> GVDNAEKGKVSNDDASVDFVAEPVKLPENQTRVAFFYDRAVPIGMLRPGQNMETTFNYQENDYRLNCLLLTPLPSFCPDSSSGPQKTKAPVQWRWVRSGGVNGANFPLMTKQDYAFLCFSPFTFYKCDLEVTVSALGTDTVASVLRWAPTGAPADVTDQLIGYTPSLGETRNPHMWLVGAGNSQVSFVVPYNSPLSVLPAAWFNGWSDFGNTKDFGVAPNADFGRLWIQGNTSASVRIRYKKMKVFCPRPTLFFPWPTPTTTKINADNPVPILELE;> DQNTEEMENLSDRVASDKAGNSATNTQSTVGRLCGYGKSHHGEHPASCADTATDKVLAAERYYTIDLASWTTSQEAFSHIRIPLPHVLAGEDGGVFGATLRRHYLCKTGWRVQVQCNASQFHAGSLLVFMAPEFYTGKGTKTGTMEPSDPFTMDTEWRSPQGAPTGYRYDSRTGFFATNHQNQWQWTVYPHQILNLRTNTTVDLEVPYVNVAPSSSWTQHANWTLVVAVLSPLQYATGSSPDVQITASLQPVNPVFNGLRHETVIAQ;> SPIPVTVREHK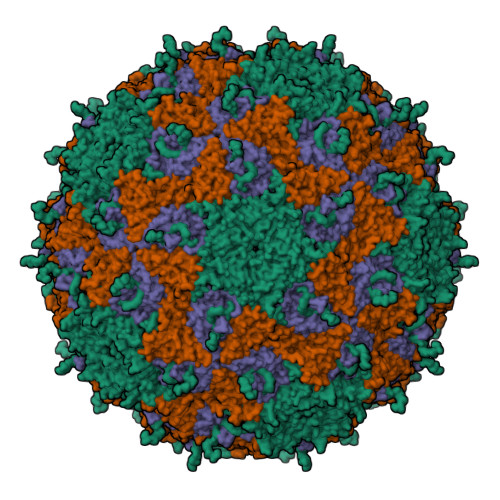GCFYSTNPDTTVPIYGKTISTPSDYMCGEFSDLLELCKLPTFLGNPNTNNKRYPYFSATNSVPATSMVDYQVALSCSCMANSMLAAVARNFNQYRGSLNFLFVFTGAAMVKGKFLIAYTPPGAGKPTTRDQAMQSTYAIWDLGLNSSFNFTAPFISPTHYRQTSYTSPTITSVDGWVTVWQLTPLTYPSGTPTNSDILTLVSAGDDFTLRMPISPTKWVPQ;> NESGNEGVIINNFYSNQYQNSIDLSASGGNAGDAPQTNGQLSNLL> VAQGPNGRALAESMNPDLLSAIQQHISIERYASVTYLAMSIWCAERELAGFYQFFDGEAKDEQSHAVHFTQYLIARSQSNDLQTLDAPRQNWDSLASLMATAFQMEADTTSSIQSVYALAERNSDTRTTVFLDPLIEAQIQSEDQFAYLLGRVKFANGDP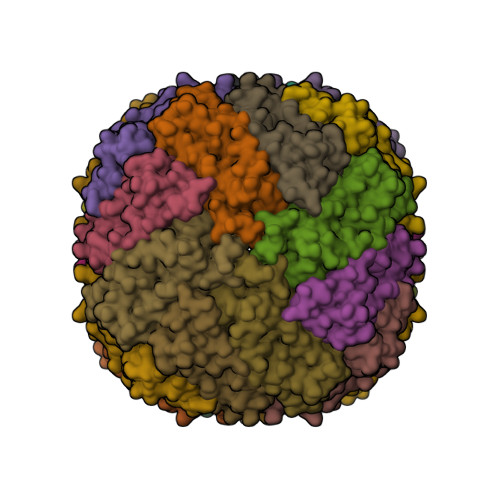TALLVIDNELRAGQTQRG>GAMGTRDDEYDYLFKVVLIGDSGVGKSNLLSRFTRNEFNLESKSTIGVEFATRSIQVDGKTIKAQIWDTAGQERYRAITSAYYRGAVGALLVYDIAKHLTYENVERWLKELRDHADSNIVIMLVGNKSDLRHLRAVPTDEARAFAEKNGLSFIETSALDSTNVEAAFQTILTEIYRIVS[3x];>[3x]GAMGSVNIPRKEKDFQGMLEYKKEDEQKLVKNLILELKPRGVAVNLIPGLPAYILFMCVRHADYLNDDQKVRSLLTSTINSIKKVLKKRGDDFETVSFWLSNTCRFLHCLKQYSGEEGFMKHNTSRQNEHCLTNFDLAEYRQVLSDLAIQIYQQLVRVLENILQPMIVSGMLEHETIQGVSGVKPTGLRKRTSSIADEGTYTLDSILRQLNSFHSVMCQHGMDPELIKQVVKQMFYIIGAITLNNLLLRKDMCSWSKGMQIRYNVSQLEEWLRDKNLMNSGAKETLEPLIQAAQLLQVKKKTDDDAEAICSMCNALTTAQIVKVLNLYTPVNEFEERVSVSFIRTIQMRLRDRKDSPQLLMDAKHIFPVTFPFNPSSLALETIQIPASLGLGFISRV

We have solved the crystal structures of the MyoVa globular tail domain in complex with Spir-2-GTBM and in complex with Rab11. The MyoV-GTD is composed of two closely apposed subdomains (SD-1 and SD-2). We have also shown that the MyoV-GTD links Spir-2 and Rab11 into a tripartite complex in vitro and in cells. The Spir:MyoV interaction contributes to the motor activation and to the coordination of the specific membrane recruitment of both actin polymerization and motor machineries required for force production powered by MyoV.

Direct interaction between the membrane anchored active Rab11 small GTPase and MyoV (MyoVa and MyoVb) globular tail domain (GTD) is necessary to target the motor to Rab11 vesicles. To gain insights into the relationship between Spir, MyoV and Rab11, we solved the crystal structure of Rab11a bound to the MyoVa-GTD. This structure confirms that Rab11a binds to the MyoVa-GTD SD-2, as previously reported for the MyoVb:Rab11a complex structure and indicates that some structural variability in Rab11a occurs upon its binding to the MyoV isoforms. The structures of MyoVa:Spir-GTBM and MyoVa:Rab11a demonstrate that the Rab11 and Spir binding sites are on opposite ends of the elongated MyoV-GTD while the GTD adopts a similar conformation in the two binary complexes. This implies that the two MyoV partners can bind to the GTD at the same time, as shown in a model of the tripartite complex. The Spir-2-GTBM (purple) binds to the SD-1 of the MyoVa-GTD (orange) and Rab11a (green, Switch-1 blue, Switch-2 red) binds to its SD-2. The MyoV motor domain and Rab11 compete for binding to the GTD since the surfaces involved in these interactions are in part overlapping (namely the H11- H12 loop). This explains why the membrane-anchored Rab11 GTPase alone is not sufficient to target the cytosolic inhibited MyoV to Rab11 positive vesicles in vivo. GST-pulldown experiments with recombinant proteins using GST-Spir-2-GTBM-SB-FYVE also confirm that MyoV serves as a linker between Spir and Rab11.>[2x]MVQQKVEVRL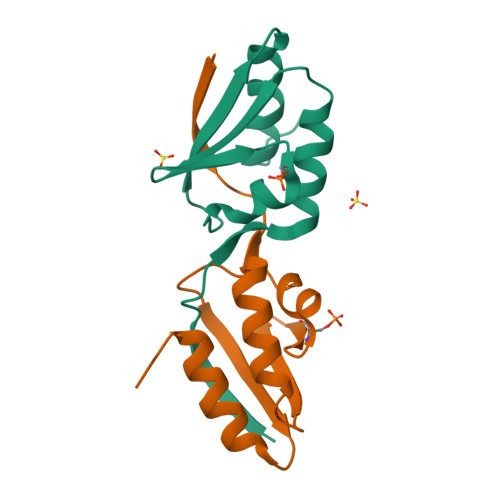KTGLQARPAALFVQEANRFTSDVFLEKDGKKVNAKSIMGLMSLAVSTGTEVTLIAQGEDEQEALEKLAAYVQEEVL>[2x]GSETDCRWDGCSQEFDSQEQLVHHINSEHIHGERKEFVCHWGGCSRELRPFK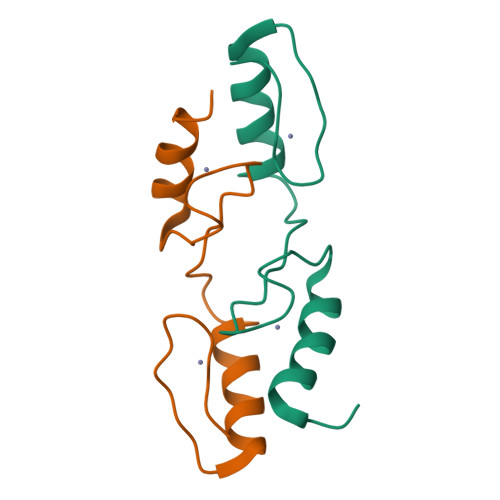AQYMLVVHMRRHTGEKPHK> MIVLFVDFDYFYAQVEEVLNPSLKGKPVVVCVFSGRFEDSGAVATANYEARKFGVKAGIPIVEAKKILPNAVYLPMRKEVYQ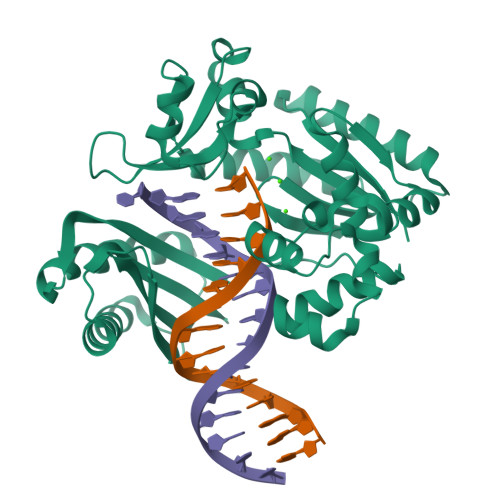QVSSRIMNLLREYSEKIEIASIDEAYLDISDKVRDYREAYNLGLEIKNKILEKEKITVTVGISKNKVFAKIAADMAKPNGIKVIDDEEVKRLIRELDIADVPGIGNITAEKLKKLGINKLVDTLSIEFDKLKGMIGEAKAKYLISLARDEYNEPIRTRVRKSIGRIVTMKRNSRNLEEIKPYLFRAIEESYYKLDKRIPKAIHVVAVTEDLDIVSRGRTFPHGISKETAYSESVKLLQKILEEDERKIRRIGVRFSKFIEAIGLDKFFDTLEHHHHHH> AQSVPYGVSQIKAPALHSQGYTGSNVKVAVIDSGIDSSHPDLKVAGGASMVPSETNPFQDNNSHGTHVAGTVAALNNSIGVLGVAPSASLYAVKVLGADGSGQYSWIINGIE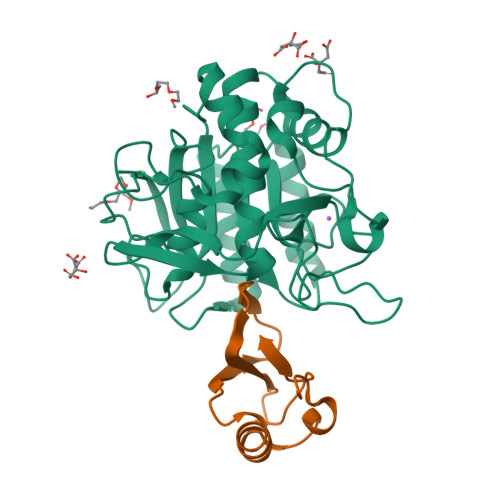WAIANNMDVINMSLGGPSGSAALKAAVDKAVASGVVVVAAAGNEGTSGSSSTVGYPGKYPSVIAVGAVDSSNQRASFSSVGPELDVMAPGVSIQSTLPGNKYGAYNGTSMASPHVAGAAALILSKHPNWTNTQVRSSLENTTTKLGDSFYYGKGLINVQAAAQHHHHHH;> MKTEWPELVGKSVEEAKKVILQDKPAAQIIVLPVGTIVTMEYRIDRVRLFVDRLDNIAQVPRVG2-[(3,5-dimethyl-1,2-oxazol-4-yl)methoxy]-~{N}-(3-methoxyphenyl)benzamide 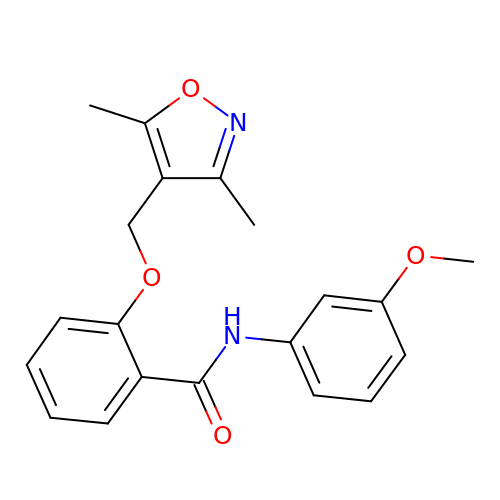| C20 H20 N2 O4 | QSTULYRIYIKOEZ-UHFFFAOYSA-N Here we used a pair of thermophilic/mesophilic acylphosphatases homologues (acylphosphatase from hyperthermophilic archaeon Pyrococcus horikoshii (PhAcP) and human common-type acylphosphatase (HuAcP)) as a model to study how local flexibility of the active site affects the enzymatic activity. Despite remarkable conservation of sequence and structure at the active site, the catalytic activity of the thermophilic PhAcP is significantly poorer as compared with its mesophilic homologue HuAcP at low temperatures. The salt-bridge between the active-site residue Arg-20 and the C-terminal carboxyl group is found only in thermophilic PhAcP but not in mesophilic HuAcP. Taken together, our data suggest that the presence of the salt-bridge between the C-terminal carboxyl group and the active-site arginine residue increases the activation energy that results in a stronger temperature dependency of the enzymatic activity.

We then questioned whether the introduction of the salt-bridge into the mesophilic homologue would result in the same observation. Firstly, the C-terminal residue of HuAcP was substituted with a glycine residue (HuG99) to engage the salt-bridge with the active-site arginine residue. Crystal structures of HuA99 and HuG99, resolved at 1.5 Å and 1.7 Å, respectively, demonstrated that they were superimposable with a Cα r.m.s.d. value of 0.17 Å. In a good agreement with our original design, the salt-bridge between the C-terminal carboxyl group of Gly-99 and Arg-23 at the active site was only detected in HuG99, but not in the pseudo-wild-type HuA99. Regarding the Arrhenius plot, both HuG99 and HuA99 exhibited straight lines that intersected also roughly at 298 K. The salt-bridge bearing variant HuG99 illustrated a steeper slope of the Arrhenius plot, i.e. a stronger temperature dependency of the enzymatic activity, as compared to that of HuA99 lacking the salt-bridge. Importantly, the activation energy (52.5±2.5 kJmol−1) for HuG99 was analogous to that for PhWT (49.1±1.4 kJmol−1), while the activation energy for HuA99 (29.5±1.9 kJmol−1) and HuWT (37.6±3.1 kJmol−1) was comparable to that for PhG91A (32.1±1.7 kJmol−1). The distance between the C-terminal carboxyl group and the guanido group of the active-site arginine residue was less than 4 Å throughout the entire simulation of PhWT and HuG99, denoting the presence of the salt-bridges in these proteins. In the simulations of the salt-bridge bearing PhWT and HuG99, the side-chains of the arginine residues populated mainly the native mtm180° rotamer conformation.

> MAEGNTLISVDYEIFGKVQGVFFRKHTQAEGKKLGLVGWVQNTDRGTVQGQLQGPISKVRHMQEWLETRGSPKSHIDKANFNNEKVILKLDYSDFQIVG> ARFEPQDIPLDIVYEDEDIIVINKPRDLVVHPGAGNPDGTVLNALLHYYPPIADVPRAGIVHRLDKDTTGLMVVAKTVPAQTRLVESLQRREITREYEAVAIGHMTAGG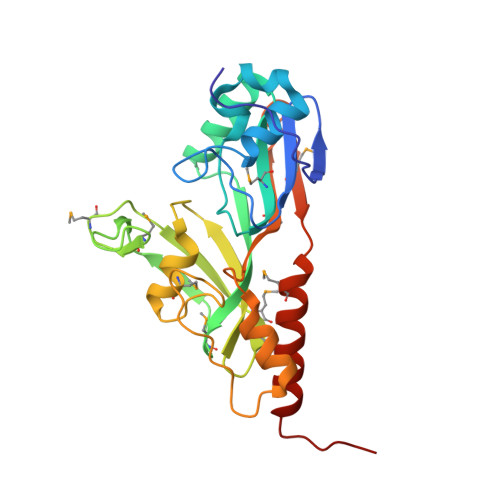TVDEPISRHPTKRTHMAVHPMGKPAVTHYRIMEHFRVHTRLRLRLETGRTHQIRVHMAHITHPLVGDPVYGGRPRPPKGASEAFISTLRKFDRQALHATMLRLYHPISGIEMEWHAPIPQDMVELIEVMRADFEEHKDEVDWL>[2x]GSKKHTGYVGLKNQGATCYMNSLLQTLFFTNQLRKAVYMMPTEGDDSSKSVPLALQRVFYELQHSDKPVGTKKLTKSFGWETLDSFMQHDVQELCRVLLDNVEN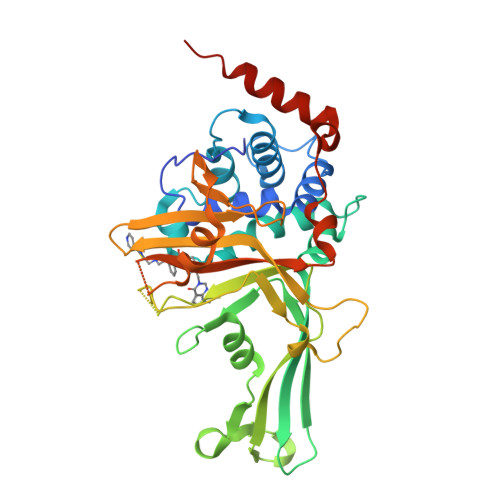KMKGTCVEGTIPKLFRGKMVSYIQCKEVDYRSDRREDYYDIQLSIKGKKNIFESFVDYVAVEQLDGDNKYDAGEHGLQEAEKGVKFLTLPPVLHLQLMRAMYDPQTDQNIKINDRFEFPEQLPLDEFLQKTDPKDPANYILHAVLVHSGDNHGGHYVVYLNPKGDGKWCKFDDDVVSRCTKEEAIEHNYGGHDDDLSVRHCTNAYMLVYIRESKLSEVLQAVTDHDIPQQLVERLQEEKRIEAQKRKERQE furanodienone | C15 H18 O2 | 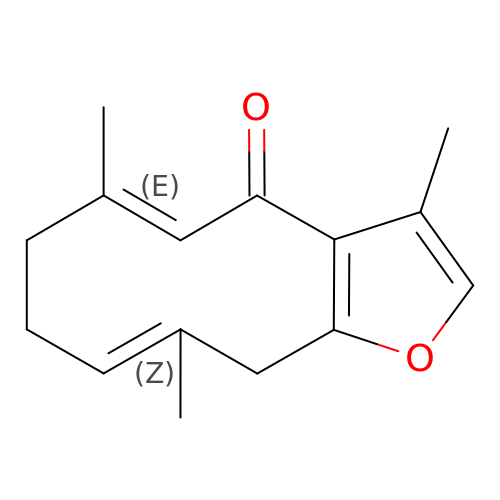XVOHELPNOXGRBQ-UHFFFAOYSA-N>[2x]SVDDEPIRLPNPMIGFGVPNEPGLITHRSLPELARGPPFFYYENVALTPKGVWETISRHLFEIPPEFVDSKYFCVAARKRGYIHNLPINNRFQIQPPPKYTIHDAFPLSKRWWPEWDKRTKLNCILTCTGSAQLTNRIRVALEPYNEEPEP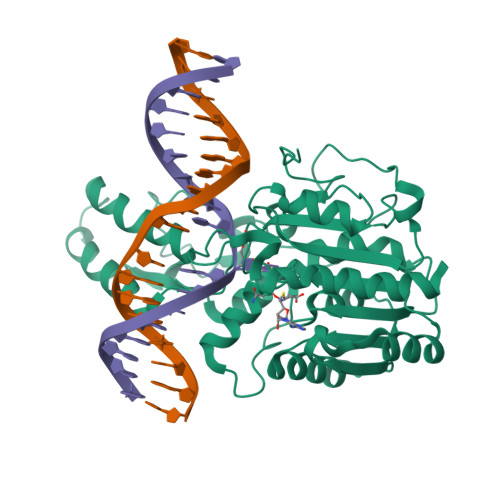PKHVQRYVIDQCKKWNLVWVGKNKAAPLEPDEMESILGFPKNHTRGGGMSRTERFKSLGNSFQVDTVAYHLSVLKPIFPHGINVLSLFTGIGGGEVALHRLQIKMKLVVSVEISKVNRNILKDFWEQTNQTGELIEFSDIQHLTNDTIEGLMEKYGGFDLVIGGSPCNNLAGGNRVSRVGLEGDQSSLFFEYCRILEVVRARMRGS>MSAKTNPGNFFEDFRLGQTIVHATPRTITEGDVALYTSLYGSRFALTSSTPFAQSLGLERAPIDSLLVFHIVFGKTVPDISLNAIANLGYAGGRFGAVVYPGDTLSTTSKVIGLRQNKDGKTGVVYVHSVGVNQWDEVVLEYIRWVMVRKRDPNAPAPETVVPDLPDSVPVTDLTVPYTVSAANYNLAHAGSNYLWDDYEVGEKIDHVDGVTIEEAEHMQATRLYQNTARVHFNLHVEREGRFGRRIVYGGHIISLARSLSFNGLANALSIAAINSGRHTNPSFAGDTIYAWSEILAKMAIPGRTDIGALRVRTVATKDRPCHDFPYRDAEGNYDPAVVLDFDYTVLM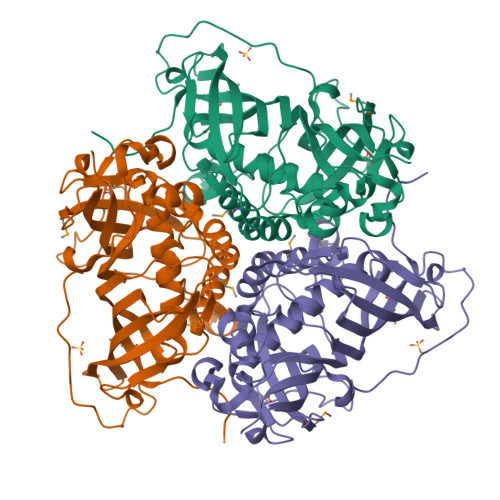PRRG[2x]>[2x]GPGHMSSSPAAPTNSANSAIALRLELLGAPVPDHAARSDFDRETDRLVAPILARQRELTRRLANRPCAADRRIQAFLDSYLDGAAAQPKLPGATLVLDQPGLARALSLPVDAT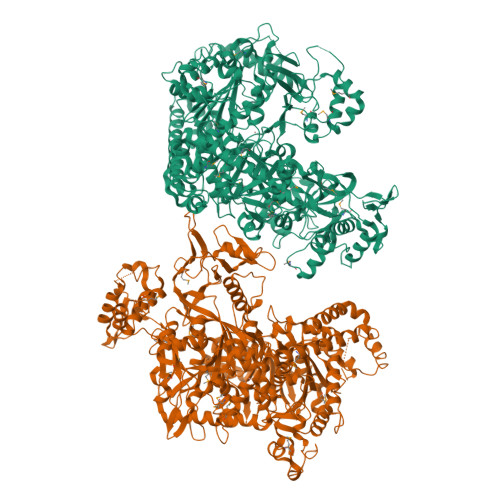SFTSDYVESYRVLSGVLHNPRNDRRTTAGVFHVAEGGLPIPDDKKAVPRDVFARVLAAAVDAPDDLMTLPWASTQADPARCFVSLLLRPVVVPEVPGFSAERSMEIRFIAPGGLVSNLDFVEGIFGNGGDPYLPENDASLAPESWTGHTGCVILAPHLTRLTKKELGLPAWEEATERQRRDGMCWRGADELYNDGKAFKLVARDERGVIVTIIADNYYGYCKKEVKTQISYSANLFGCVEEEHSGGALAFPRYNLGQEYTDVHTPAGATVERVLARNPGRFEARADGSAVLLDDDGRPDEGIVLVPAGAHFSMRTQTVTWDRADGREASIPLLADRVYIAPGGYRVHAKHREGDATQWHLVGTAPWATQAHKPATVSGGGKSEISKSLLDAFVFGEAYVGDVDADLDAVQKILDGNYADRFVDPANKSAHHRPILSERRSLGSVIKLLTPSSMYTEEYNAFLESIPAHIKELIFTVKRYYQPGWGADWRSHFSVGIINGRKGNSLRLDGEVIKVNMLRVGFEDDGAWRLLSLRPDFSPAAKVQTEDDITSSIVAPGGLESTAGSSVSRKFVTNCESLLFQRPDDAIVRGYDKQTERDMSGTGLFISNYQPLTPADARAMVADAPGLSRFTEPMQELVRRAAAIPEAADPREETYWTSTANPRLVGGAPTRNPRYLQVRPDIANPRDVALADLSIHLYRDAPLAAPARHGVDVVAAGRRNNPPEPGVPALCAYNPLHYMELPELFMEFISSMTGKSPSTTGAGSEGALTKSPFNALPPVYDLNAALLSYALGGYDGWLSSAGYIGPKVKVAHDISLLVPEIFSRMTPQERDARALIEAGYLERLEDFDHEGRRIEASRLGYRMNAAFATAYFGRIFLHPDVVFTEEMLRPELQDPAIFADSVEVIVATHRAVAKHYVDDGSIQWAVPPLKALLEIMYSGRSEEGWTLSSPELRALFERENILASDWYAERVDAKVERDRKQAESAIAALTRFTTTQGNEEVTERLDIEGRLASARAWLDEVTSPAYRAHLVGTLGLQPSLA>[4x]GSHMLNIQNYSASPHPGIVAERPQTPSASEHVETAVVPSTTEHRGTDIISLSQAATKIHQAQQTLQSTPPISEENNDERTLARQQLTSSLNALAKSGVSLSAEQNENLRSAFSAPTSALFSASPMAQPRTTISDAEIWDMVSQNISAIGDSYLGVYENVVAVYTDFYQAFSDILSKMGGWLLPGKDGNTVKLDVTSLKNDLNSLVNKYNQINSNTVLFPAQSGSGVKVATEAEARQWLSELNLPNSCLKSYGSGYVVTVDLTPLQKMVQDIDGLGAPGKDSKLEMDNAKYQAWQSGFKAQEENMKTTLQTLTQKYSNANSLYDNLVKVLSSTISSSLETAKSFLQG

Bacterial infections including Salmonellosis and Shigellosis affect millions of people every year. These bacteria use a T3SS to secrete virulence factors to manipulate host cells. The T3SS is a multi-component system that forms a continuous protein transport channel through the two bacterial membranes and the periplasmatic space that extends into the surrounding medium by a needle structure. Tip proteins, which bind to the distal end of the T3SS needle, are thought to play an important role in this process. SipD from S. typhimurium, IpaD from Shigella flexneri and BipD from Burkholderia mallei are tip proteins that are thought to interact with their corresponding needle subunits PrgI, MxiH and BsaL, respectively, to make the needle tip complex.

We solved the X-ray crystal structure of SipD, the needle tip protein of S. typhimurium at 3.0 Å resolution. The crystal contained 4 copies of SipD in the asymmetric unit with structural information for 306 of 343 amino acids. Here we report structural features of SipD chain A, which, compared with chains B to D, showed continuous electron density for most amino acids. SipD is predominantly α-helical folded and can be divided in three structurally different domains. The central domain, domain 2, (green in Figure 1) adopted a coiled coil structure with two helices of 47 and 52 amino acids length, respectively. The bending of the coiled coil of domain 2 allowed us to distinguish between a concave and a convex surface. Domain 2 is joined to domain 3, an α/β-structure (yellow in Figure 1). Domain 3 is in contact with the convex surface provided by the coiled coil of the central domain. Domain 2 and 3 of SipD share high sequence homology and similar three dimensional structure to the orthologs from S. flexneri (r.m.s. deviation 1.3 Å with IpaD) or B. mallei (r.m.s. deviation 2.2 Å with BipD). Notably, amino acids involved in intramolecular contacts are identical or highly conserved in all three orthologs, suggesting functional relevance in T3SS tip proteins.> MRNLDFIDSFIPTEGKYIRVMDFYNSEYPFCIHAPSAPNGDIMTEICSRENNQYF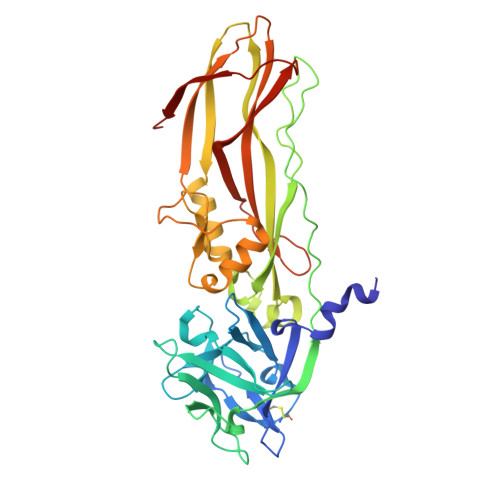IFFPTDDGRVIIANRHNGSVFTGEATSVVSDIYTGSPLQFFREVKRTMATYYLAIQNPESATDVRALEPHSHELPSRLYYTNNIENNSNILISNKEQIYLTLPSLPENEQYPKTPVLSGIDDIGPNQSEKSIIGSTLIPCIMVSDFISLGERMKTTPYYYVKHTQYWQSMWSALFPPGSKETKTEKSGITDTSQISMTDGINVSIGADFGLRFGNKTFGIKGGFTYDTKTQITNTSQLLIETTYTREYTNTENFPVRYTGYVLASEFTLHRSDGTQVNTIPWVALNDNYTTIARYPHFASEPLLGNTKIITDDQN> CPEQDKYRTITGMCNNRRSPTLGASNRAFVRWLPAEYEDGFSLPYGWTPGVKRNGFPVALARAVSNEIVRFPTDQLTPDQERSLMFMQWGQLLDHDLDFTPEPAARASFVTGVNCETSCVQQPPCFPLKIPPNDPRIKNQADCIPFFRSCPACPGSNITIRNQINALTSFVDASMVYGSEEPLARNLRNMSNQLGLLAVNQRFQDNGRALLPFDNLHDDPCLLTNRSARIPCFLAGDTRSSEMPELTSMHTLLLREHNRLATELKSLNPRWDGERLYQEARKIVGAMVQIITYRDYLPLVLGPTAMRKYLPTYRSYNDSVDPRIANVFTNAFRYGHTLIQPFMFRLDNRYQPMEPNPRVPLSRVFFASWRVVLEGGIDPILRGLMATPAKLNRQNQIAVDE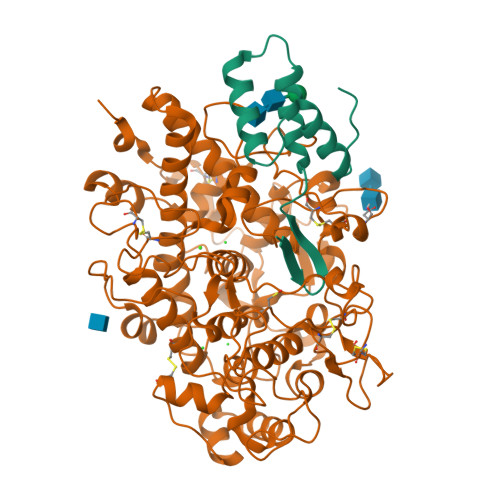IRERLFEQVMRIGLDLPALNMQRSRDHGLPGYNAWRRFCGLPQPETVGQLGTVLRNLKLARKLMEQYGTPNNIDIWMGGVSEPLKRKGRVGPLLACIIGTQFRKLRDGDRFWWENEGVFSMQQRQALAQISLPRIICDNTGITTVSKNNIFMSNSYPRDFVNCSTLPALNLASWREA;> GSTKVYSQNGLVLHDDANFLEHELSYIDVLLDKNADQATKDNLRSYFADKGLHSIKDIINKAKQDGFDVSK> GPLGSMSEEQVAQDTEEVFRSYVFYRHQQEQEAEGVAA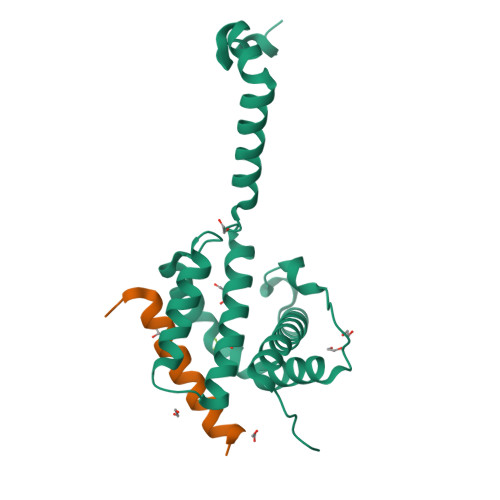PADPEMVTLPLQPSSTMGQVGRQLAIIGDDINRRYDSEFQTMLQHLQPTAENAYEYFTKIATSLFESGINWGRVVALLGFGYRLALHVYQHGLTGFLGQVTRFVVDFMLHHSIARWIAQRGGWVAALNLGNG;> DMRPEIRIAQELRRIGDEFNATYAR> GAGCGACCTGTACGGACATCACATGCTGAGT;> AACCTACCTGGCAGGACGACT;> CACGAGCCTGATCGGACAAGA;> TTAGTCGTGGCTCG;> TGTCTTGTGGTCGC;> TCACTCAGCATGTGATGTGGTAGG;> TACACCGA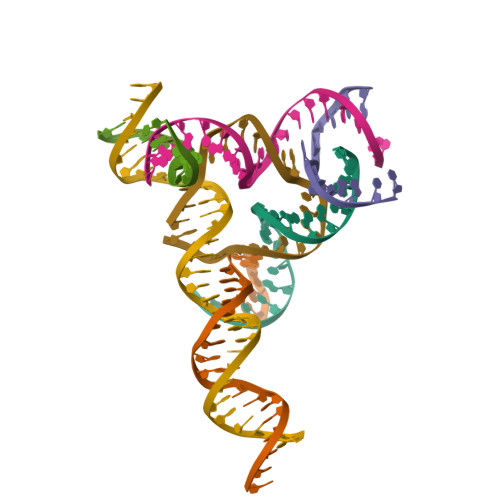TCACCTGCCACCG>MKLAYSLDATASFLNFVSSKKTHVLETHRFDVLSGGISTAGEAQLVIDLNSVNTGIDVRNGRMRDYLFETATYSVATVTVPVDLAAVAGLAVGEDMLVDVSATLDLHGVPGVIDTQLNVQRLSATRIMVQ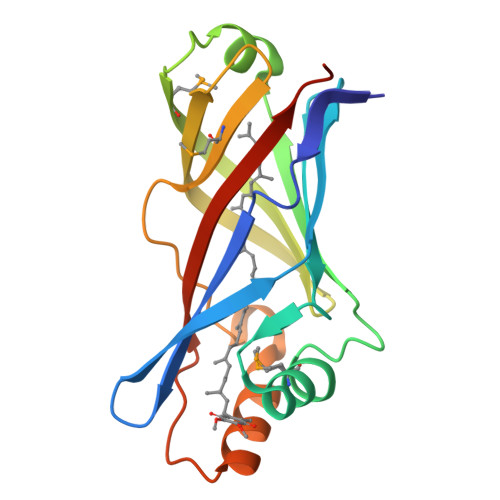NQSPLLIKAADYSLEAGIETLRNLASLNVISTTVPVDFVLFYEAPHHHHHH[2x]Prohibitins are a highly conserved family of proteins that have been implicated in a variety of functions including mitochondrial stress signalling and housekeeping, cell cycle progression, apoptosis, lifespan regulation and many others. The human prohibitins prohibitin 1 and prohibitin 2 have been proposed to act as scaffolds within the mitochondrial inner membrane, but their molecular organization has remained elusive. Here we determined the molecular organization of the human prohibitin complex within the mitochondrial inner membrane using an integrative structural biology approach combining quantitative western blotting, cryo-electron tomography, subtomogram averaging and molecular modelling. The proposed bell-shaped structure consists of 11 alternating prohibitin 1 and prohibitin 2 molecules.

Finally, we re-extracted the subtomograms at 2.5 Å pixel size for automated 3D refinement with implied C11 symmetry, resulting in a final cryo-EM map of the prohibitin assembly at 16.3 Å resolution (FSC, 0.143 criterion). The final cryo-EM map reveals a circular bell-shaped structure that is embedded into the lipid bilayer with a diameter of 190.2 Å directly above the lipid bilayer. The whole bell has a height of 84.0 Å measured from the lipid bilayer to the top of the particle and a narrowed top with a diameter of 89.0 Å. Notably, the map reveals a large empty cavity on top of the bilayer enclosed by the bell. As the structures of PHB1 and PHB2 have yet to be solved experimentally, we relied on AlphaFold2 to predict the structures of full length PHB1 and PHB2. Numerous possible arrangements were tested but we found that each of the 11 densities in the cryo-EM map can accommodate only one prohibitin molecule. The final molecular model comprises 11 monomeric PHB molecules forming a bell-shaped assembly. On the contrary, adjacent PHB C-termini interact more strongly and stabilize the centre of the bell top. We also identified self-linked peptides where the same residues were crosslinked in overlapping peptides, thereby indicating the occurrence of homomeric interactions. Interestingly, these self-links only satisfied the distance constraint at the PHB1–PHB1 or PHB2–PHB2 (Fig. 4b(i,ii)) interfaces and were violated when mapped to the rest of the PHB heteromeric structure with alternating PHB1 and PHB2 subunits.

>[6x]MAAKVFESIGKFGLALAVAGGVVNSALYNVDAGHRAVIFDRFRGVQDIVVGEGTHFLIPWVQKPIIFDCRSRPRNVPVITGSKDLQNVNITLRILFRPVASQLPRIFTSIGEDYDERVLPSITTEILKSVVARFDAGELITQRELVSRQVSDDLTERAATFGLILDDVSLTHLTFGKEFTEAVEAKQVAQQEAERARFVVEKAEQQKKAAIISAEGDSKAAELIANSLATAGDGLIELRKLEAAEDIAYQLSRSRNITYLPAGQSVLLQLPQ;>[5x]MAQNLKDLAGRLPAGPRGMGTALKLLLGAGAVAYGVRESVFTVEGGHRAIFFNRIGGVQQDTILAEGLHFRIPWFQYPIIYDIRARPRKISSPTGSKDLQMVNISLRVLSRPNAQELPSMYQRLGLDYEERVLPSIVNEVLKSVVAKFNASQLITQRAQVSLLIRRELTERAKDFSLILDDVAITELSFSREYTAAVEAKQVAQQEAQRAQFLVEKAKQEQRQKIVQAEGEAEAAKMLGEALSKNPGYIKLRKIRAAQNISKTIATSQNRIYLTADNLVLNLQDESFTRGSDSLIKGKK> MRNLDFIDSFIPTEGKYIRVMDFYNSEYPFCIHAPSAPNGDIMTEICSRENNQYFIFFPTDDGRVIIANRHNGSVFTGEATSVVSDIYTGSPLQFFREVKRTMATYYLAIQNPESATDVRALEPHSHELPSRLYYTNNIENNSNILISNKEQIYLTLPSLPENEQYPKTPVLSGIDDIGPNQSEKSIIGSTLIPCIMVSD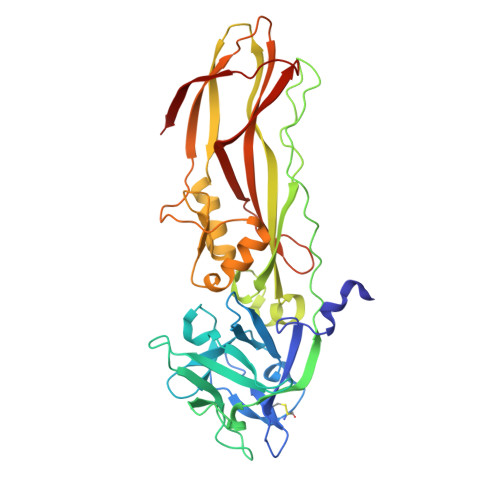FISLGERMKTTPYYYVKHTQYWQSMWSALFPPGSKETKTEKSGITDTSQISMTDGINVSIGADFGLRFGNKTFGIKGGFTYDTKTQITNTSQLLIETTYTREYTNTENFPVRYTGYVLASEFTLHRSDGTQVNTIPWVALNDNYTTIARYPHFASEPLLGNTKIIT> CSELIQASSRITTCSTEGVNTKCRLSGTALIRAGSVGAEACLMLKGVKEDQTKFLKIKTVSSELSCREGQSYWTGSFSPKCLSSRRCHLVGECHVNRCLSWRDNETSAEFSFVGESTTMRENK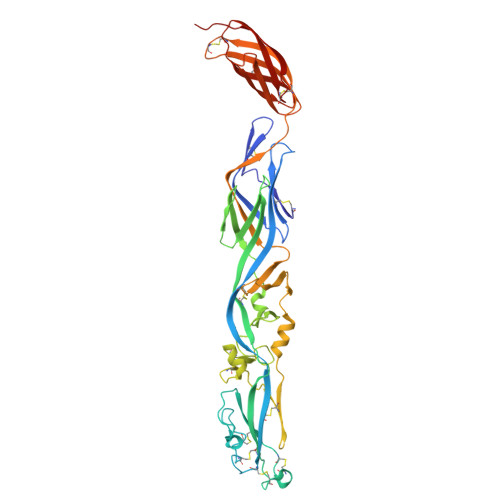CFEQCGGWGCGCFNVNPSCLFVHTYLQSVRKEALRVFNCIDWVHKLTLEITDFDGSVSTIDLGASSSRFTNWGSVSLSLDAEGISGSNSFSFIESPGKGYAIVDEPFSEIPRQGFLGEIRCNSESSVLSAHESCLRAPNLISYKPMIDQLECTTNLIDPFVVFERGSLPQTRNDKTFAASKGNRGVQAFSKGSVQADLTLMFDNFEVDFVGAAVSCDAAFLNLTGCYSCNAGARVCLSITSTGTGSLSAHNKDGSLHIVLPSENGTKDQCQILHFTVPEVEEEFMYSCDGDERPLLVKGTLIAID(4~{S})-5-[4-[[4-(2-ethyl-2-oxidanyl-butoxy)-3-methyl-phenyl]-methyl-propyl-silyl]-2-methyl-phenoxy]-4-oxidanyl-pentanoic acid 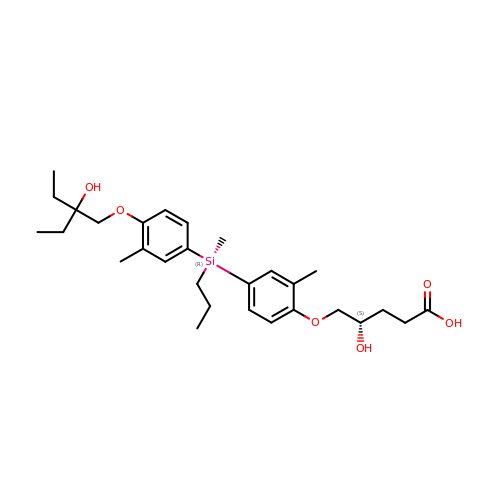| C29 H44 O6 Si | QIPUEXXIUNZLGD-RJVOLCHMSA-N>[4x]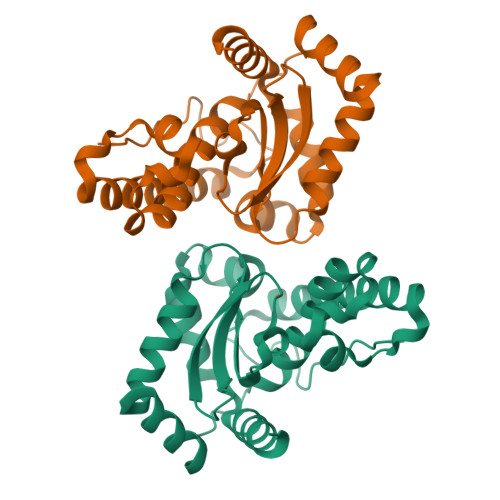MAILLPDLPYAYDALEPYIDAETMTLHHDKHHATYVANANAALEKHPEIGENLEVLLADVEQIPADIRQSLINNGGGHLNHALFWELLSPEKTKVTAEVAAAINEAFGSFDDFKAAFTAAATTRFGSGWAWLVVDKEGKLEVTSTANQDTPISQGLKPILALDVWEHAYYLNYRNVRPNYIKAFFEVINWNTVARLYAEALTLEHHHHHH>MAASLPSTLSFSSAPDEIQHPQIKFSEWKFKLFRVRSFEKAPEEAQKEKDSSEGKPYLEQSPVVPEKPGGQNSILTQRALKLHPKFSKKFHADGKSSDKAVHQARLRHFCRICGNRFKSDGHSRRYPVHGPVDAKTQSLFRKKEKRVTSWPDLIARIFRIDVKADVDSIHPTEFCHDCWSIMHRKFSSSHSQVYFPRKVTVEWHPHTPSCDICFTAHRGLKRKRHQPNVQLSKKLKTVLNHARRDRRKRTQARVSSKEVLKKISNCSKIHLSTKLLAVDFPAHFVKSISCQICEHILADPVETSCKHLFCRICILRCLKVMGSYCPSCRYPCFPTDLESPVKSFLNILNSLMVKCPAQDCNEEVSLEKYNHHVSSHKESKETLVHINKGGRPRQHLLSLTRRAQKHRLRELKIQVKEFADKEEGGDVKAVCLTLFLLALRARNEHRQADELEAIMQGRGSGLQPAVCLAIRVNTFLSCSQYHKMYRTVKAITGRQIFQPLHALRNAEKVLLPGYHPFEWQPPLKNVSSRTDVGIIDGLSGLASSVDEYPVDTIAKRFRYDSALVSALMDMEEDILEGMRSQDLDDYLNGPFTVVVKESCDGMGDVSEKHGSGPAVPEKAVRFSFTVMRITIEHGSQNVKVFEEPKPNSELCCKPLCLMLADESDHETLTAILSPLIAEREAMKSSELTLEMGGIPRTFKFIFRGTGYDEKLVREVEGLEASGSVYICTLCDTTRLEASQNLVFHSITRSHAENLQRYEVWRSNPYHESVEELRDRVKGVSAKPFIETVPSIDALHCDIGNAAEFYKIFQLEIGEVYKHPNASKEERKRWQATLDKHLRKRMNLKPIMRMNGNFARKLMTQETVDAVCELIPSEERHEALRELMDLYLKMKPVWRSSCPAKECPESLCQYSFNSQRFAELLSTKFKYRYEGKITNYFHKTLAHVPEIIERDGSIGAWASEGNQSGNKLFRRFRKMNARQSKCYEMEDVLKHHWLYTSKYLQKFMNAHNALKSSGFTMNSKETLGDPLGIEDSLESQDSMEF[2x];>MSLQMVTVGHNIALIQPGFSLMNFDGQVFFFGQKGWPKRSCPTGVFHFDIK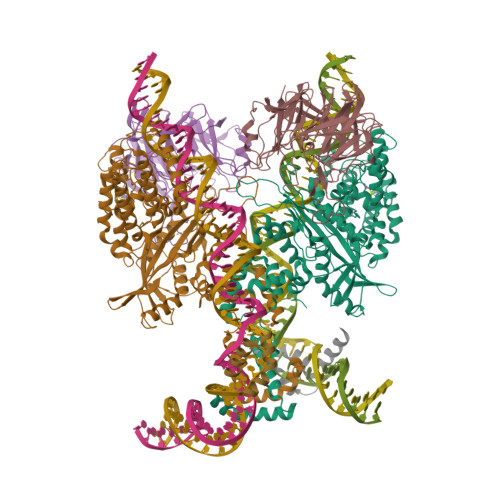QNHLKLKPAIFSKDSCYLPPLRYPATCSYKGSIDSDKHQYIIHGGKTPNNELSDKIYIMSVACKNNKKVTFRCTEKDLVGDVPEPRYGHSIDVVYSRGKSMGVLFGGRSYMPSTQRTTEKWNSVADCLPHVFLIDFEFGCATSYILPELQDGLSFHVSIARNDTVYILGGHSLASNIRPANLYRIRVDLPLGTPAVNCTVLPGGISVSSAILTQTNNDEFVIVGGYQLENQKRMVCSLVSLGDNTIEISEMETPDWTSDIKHSKIWFGSNMGNGTIFLGIPGDNKQAMSEAFYFYTLRCSEEDLSEDQKIVSNSQTSTEDPGDSTPFEDSEEFCFSAEATSFDGDDEFDTYNEDDEDDESVTGYWITCCPTCDVDINTWVPFYSTELNKPAMIYCSHGDGHWVHAQCMDLEERTLIHLSEGSNKYYCNEHVQIARALQTPKRNPPLQKPPMKSLHKKGSGKVLTPAKKSFLRRLFD[2x];>[2x]MGKGDPKKPRGKMSSYAFFVQTCREEHKKKHPDASVNFSEFSKKCSERWKTMSAKEKGKFEDMAKADKARYEREMKTYIPPKGETKKKFKDPNAPKRPPSAFFLFCSEYRPKIKGEHPGLSIGDVAKKLGEMWNNTAADDKQPYEKKAAKLKEKYEKDIAAYR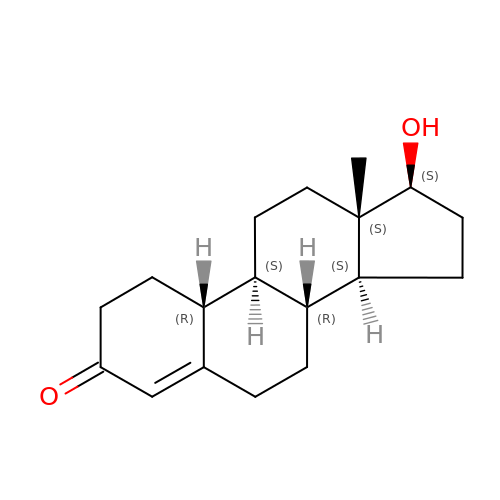(8~{R},9~{S},10~{R},13~{S},14~{S},17~{S})-13-methyl-17-oxidanyl-2,6,7,8,9,10,11,12,14,15,16,17-dodecahydro-1~{H}-cyclopenta[a]phenanthren-3-one | C18 H26 O2 | NPAGDVCDWIYMMC-IZPLOLCNSA-N>MKENKLDYIPEPMDLSLVDLPESLIQLSERIAENVHEVWAKARIDEGWTYGEKRDDIHKKHPCLVPYDELPEEE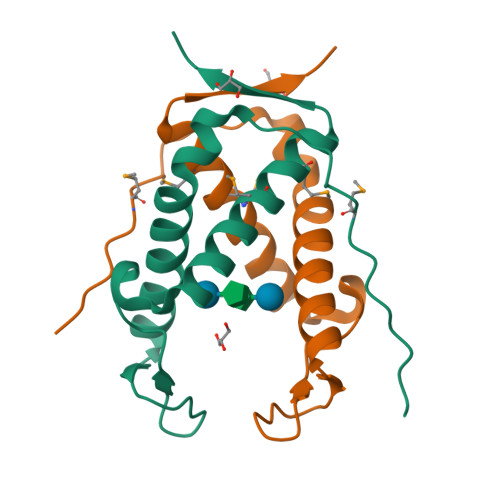KEADRNTAMNTIKMVKKLGFRIEKED[6x]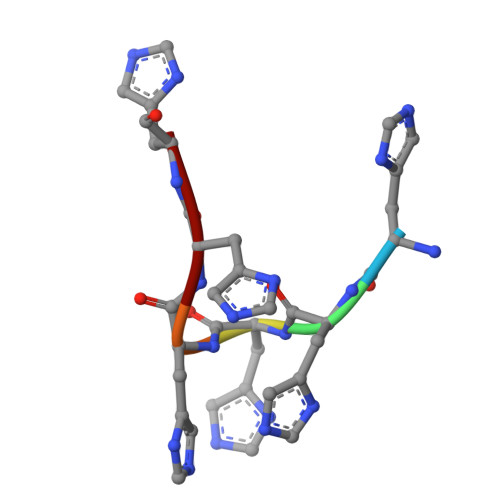> HHHHHH> GAMRQLAVIPPMLYDADQQRIKFINMNGLMADPMKVYKDRQVMNMWSEQEKETFREKFMQHPKNFGLIASFLERKTVAECVLYYYLTKK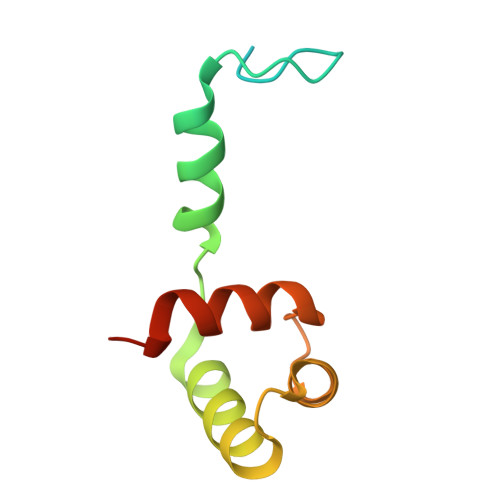NENYK> AVCPDGTRVSHAACCAFIPLAQDLQETIFQNECGQDAHEVIRLTFHDAIAISRSQGPKAGGGADGSMLLFPTVEPNFSANNGIDDSVNNLIPFMQKHNTISAADLVQFAGAVALSNCPGAPRLEFLA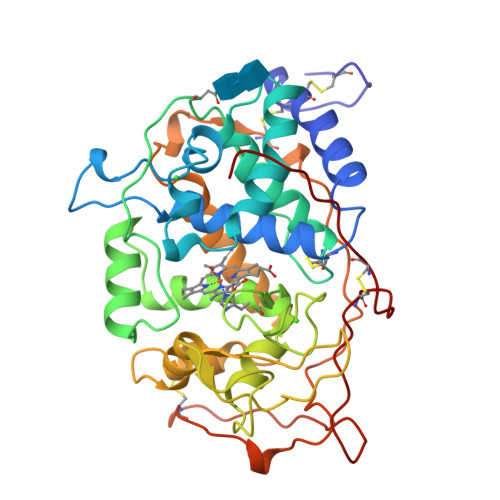GRPNKTIAAVDGLIPEPQDSVTKILQRFEDAGGFTPFEVVSLLASHSVARANKVDQTIDAAPFDSTPFTFDTQVFLEVLLKGVGFPGSANNTGEVASPLPLGSGSDTGEMRLQSDFALAHDPRTACIWQGFVNEQAFMAASFRAAMSKLAVLGHNRNSLIDCSDVVPVPKPATGQPAMFPASTGPQDLELSCPSERFPTLTTQPGASQSLIAHCPDGSMSCPGVQFNGPA> GSHMLETFNKITPNLAEFAFSLYRQLAHQSNSTNIFFSPVSIATAFAMLSLGTKADTHDEILEGLNFNLTEIPEAQIHEGFQELLRTLNQPDSQLQLTTGNGLFLSEGLKLVDKFLEDVKKLYHSEAFTVNFGDTEEAKKQINDYVEKGTQGKIVDLVKELDRDTVFALVNYIFFKGKWERPFEVKDTEEEDFHVDQVTTVKVPMMKRLGMFNIQHAKKLSSWVLLMKYLGNATAIFFLPDEGKLQHLENELTHDIITKFLENEDRRSASLHLPKLSITGTYDLKSVLGQLGI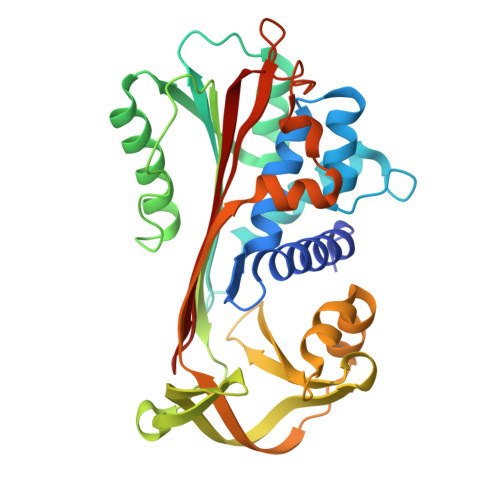TKVFSNGADLSGVTEEAPLKLSKAVHKAVLTIDEKGTEAAGADDDEAIPR> MTPTTNNKRINFASIKNPLFYPDFLEVQLKSFHDFLQLDTPPERRKKEGLYKVFAENFPITDTRNNFVLEFLDYYIDPPKYSIEECLSRGLTYSVPLKAKLKLYCTDPDHEDFATVIQDVFLGPIPYMTSSGTFVINGAERVIVSQLHRSPGVFFGQSLHTNGTKLYSARIIPFKGSWIEFATDINNVMYAYIDRKKKLPVTTLLRAIGFEADKDILDIFNLADEVKVTKANLKKCIGRKLAARVINTYIDDLSDEDTGEVVSMERITVVVDREVELTEDNIEAILNSNAQTILLHRNDSNTSDYSIIFNTLQKDPCNSEKEALYYVYRQLRNAEPADDASAREVITNLFFSDKRYDLGDVGRYRINKKLNLNIDPDIKVLTNEDIIEIIKYLIELVNSKASVDDIDHLSNRRVRTVGEQLYNQFGIGLARMARTVRDRMNVRDNEVFTPIDLVNAKTISSVVNSFFGTNALSQFMDQTNPLAEITHKRRLSALGPGGLSRERAGFEVRDVHYTHYGRLCPIETPEGPNIGLISSLCVYAKISDLGFITTPYREVKNGKVDFSDNGLKYYTAEEEEEKTVAQGNAPLDENGRFVRERVKARYESDFPLVTPDEVDLMDVSPTQIASIAAALIPFLEHDDANRALMGSNMMRQAVPLLRPESPIVGTGIEGKLVKDSRTQIVAERGGEVVFVDAS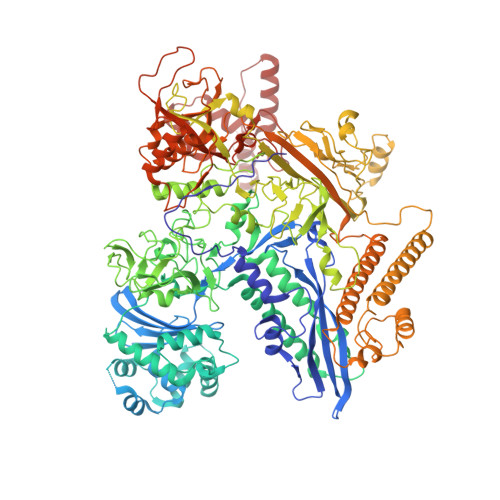CIKIRYDRTADEEFVSFDDAIVTYYLPKYRKTNQSTTIDLHPICSKGDRVEAGQILTEGYSTQGGELALGRNVQVAYMPWKGYNYEDAIVLNERMVREDFFTSVHVDEYILEVRETKRGLEELTSDIPNVSEDATRDLDENGIVRIGAHIEPGDILIGKITPKGESDPTPEEKLLRAIFGDKAGDVKDASLKATPSLRGVVIDTKLFSKAAKKKSRTSTKEAVSKLDETYAKRQQQLHERLIEKLTELTKGKTCCGVKDYLNVELIKAGSKFTKKDLEALDFNVIQLSDWTNDAHTNELIKAVAVNYLKHSKEIEAELRRRKLDETIGDELPAGIVQMAKVYIAKKRKIQVGDKMAGRHGNKGIVSKIVRQEDMPFLADGTPVDICLNPLGVPSRMNLGQIFEAVLAWAGRKMNVKFATPIFDGASLNDMNEWTDKAGLPRDGKTYLYDGGTGERFDQPATVGVTYFLKLGHMVDDKMHARSIGPYSLITQQPLGGKAQFGGQRFGEMEVWALEAFGASHILQEILTVKSDDVVGRSKAYEAIVKGDPMPTPGIPESLNVLLHELKGLGLSFSLD> SMHLICQSGDVLSARYEIVDTLGEGAFGKVVECIDHKAGGRHVAVKIVKNVDRYCEAARSEIQVLEHLNTTDPNSTFRCVQMLEWFEHHGHICIVFELLGLSTYDFIKENGFLPFRLDHIRK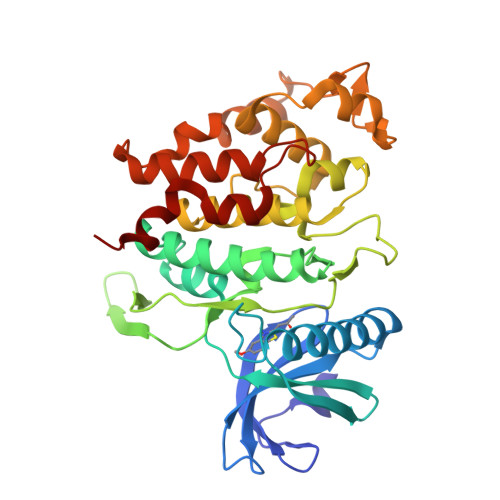MAYQICKSVNFLHSNKLTHTDLKPENILFVQSDYTEAYNPKIKRDERTLINPDIKVVDFGSATYDDEHHSTLVSTRHYRAPEVILALGWSQPCDVWSIGCILIEYYLGFTVFPTHDSKEHLAMMERILGPLPKHMIQKTRKRKYFHHDRLDWDEHSSAGRYVSRACKPLKEFMLSQDVEHERLFDLIQKMLEYDPAKRITLREALKHPFFDLLKKSI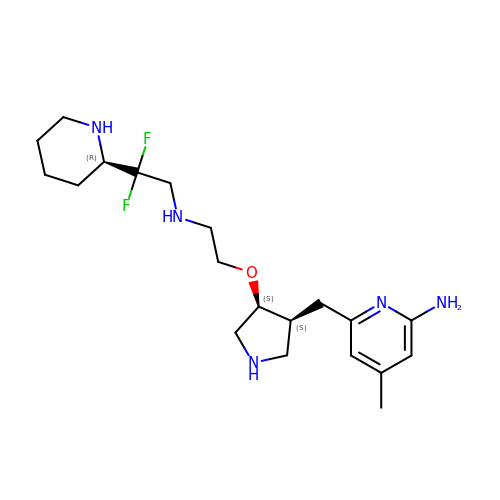6-({(3S,4S)-4-[2-({2,2-difluoro-2-[(2R)-piperidin-2-yl]ethyl}amino)ethoxy]pyrrolidin-3-yl}methyl)-4-methylpyridin-2-amine | C20 H33 F2 N5 O | PYDITBVREMCKIX-CGTJXYLNSA-N> CTCTTCTTC;> GAAG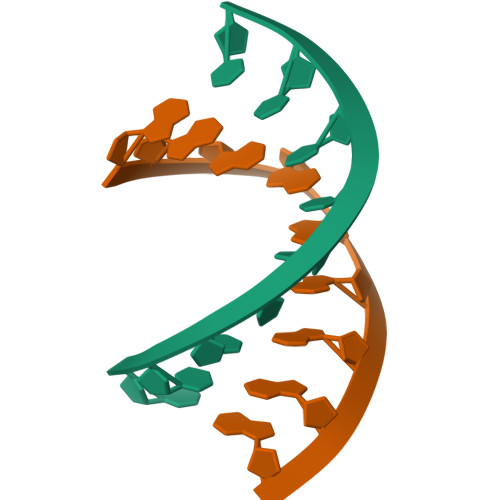AAGAG> HHHHHHMQAQVFRVPMSNPADVSGVAKLIDEGVIRAEEVVCVLGKTEGNGCVNDFTRGYTTLAFKVYFSEKLGVSRQEVGERIAFIMSGGTEGVMAPHCTIFTVQKTDNKQKTAAEGKRLAVQQIFTREFLPEEIGRMPQVTETADAVRRAMREAGIADASDVHFVQVKCPLLTAGRMHDAVERGHTVATEDTYESMGYSRGASALGIALALGEVEKANLSDEVITADYSLYSSVASTSAGIELMNNEIIVMGNSRAWGGDLVIGHAEMKDAIDGAAVRQALRDVGCCENDLPTVDELGRVVNVFAKAEASPDGEVRNRRHTMLDDSDINSTRHARAVVNAVIASIVGDPMVYVSGGSEHQGPAGGGPVAVIARTA

Cyanuric acid hydrolases are members of a protein family containing only themselves and the barbiturase enzymes, they are found only in microorganisms, and are present in approximately 0.3% of sequenced prokaryotic genomes. The enzyme is proposed to catalyze an opening of the s-triazine ring via a nucleophilic serine residue that is activated by a nearby lysine, a mechanistic motif known as a serine-lysine dyad. TrzD is a 370 amino acid, ~39.5 kDa protein that exhibits a complex α/β structure characteristic of the cyanuric acid hydrolase family enzyme. The three structurally homologous domains form a pseudo-three-fold internal symmetry in the TrzD monomer.

The product-bound structure was refined to a resolution of 2.19 Å, with Rwork and Rfree values of 0.15 and 0.20, respectively, yielding high quality electron density maps. An examination of the active site revealed, unexpectedly, the active site lysine residue in domain 2 (Lys163), that in other structures paired with the proposed nucleophilic serine, exhibited a significant displacement out of the active site, and opening a clear channel from the buried active site to the protein surface. Moreover, the difference Fourier map (Fo − Fc) clearly showed electron density corresponding to two CO2 molecules and Lys163 within the TrzD structure. As expected, since CO2 is a co-product, one is located in the active site, while the second one was observed at the interface of domain 2 and 3, proposed here as the exit channel for product release. The CO2 molecule is stabilized by H-bonds with the side chain oxygen of Ser82, Ser233 and Ser349 (~2.9 Å), and the backbone amide nitrogen of Gly350 (3.3 Å), backbone carbonyl oxygen of Gly83 and also with a side chain nitrogen of Arg330. The oxygen atoms of the CO2 molecule were stabilized by two paired H-bonds with the side chains of Arg51 and Glu237 from domain 1 and domain 2, respectively, with additional stabilization by the hydrophobic residue Ile236 backbone amide N and Glu237 backbone amide N. The present structure has an Mg+2 bound and makes 6-contacts with neighboring residues and one with a solvent molecule (2.8 Å). In the TrzD structure uniquely, Lys163, which is conserved in all cyanuric acid hydrolases, was re-oriented toward the surface, opening up an exposed channel between the domain 1 and 2 interface. Here we propose this to be the product exit channel. In silico, carbon dioxide remained bound, thus revealing the exit channel. By this model, domain 2 lysine’s role in catalysis is not limited to activating catalytic serine to open the ring but also guides products towards the exit channel.> SYYAVAVVKKGTDFMIKDLRGKTSCHTGLGRSAGWNIPIGTLIHRGDIEWEGIESGSVEQAVAKFFSASCVPGATTEQKLCRQCKGDAKTKCLRNAPYSGYSGAFQCLKDGKGDVAFVKHTTVQENAPEEKDE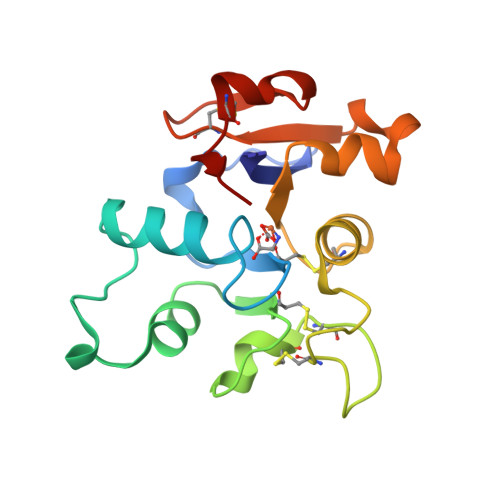YELLCLDGTRQPVDSYKTCNWARVAA> GGGFCTSAGALWIYPTNCPVRDYQLHISRAALFCNTLVCLPTGLGKTFIAAVVMYNFYRWFPSGKVVFMAPTKPLVTQQIEACYQVMGIPQSHMAEMTGSTQASTRKEIWCSKRVLFLTPQVMVNDLSRGACPAAEIKCLVIDEAHKALGNYAYCQVVRELVKYTNHFRILALSATPGSDIKAVQQVITNLLIGQIELRSEDSPDILTYSHERKVEKLIVPLGEELAAIQKTYIQILESFARSLIQRNVLMRRDIPNLTKYQIILARDQFRKNPSPNIVGIQQGIIEGEFAICISLYHGYELLQQMGMRSLYFFLCGIMDGTKGMTRSKNELGRNEDFMKLYNHLECMFARTRSTSANGISAIQQGDKNKKFVYSHPKLKKLEEVVIEHFKSWNAENTTEKKRDETRVMIFSSFRDSVQEIAEMLSQHQPIIRVMTFVGHASGKSTKGFTQKEQLEVVKQFRDGGYNTLVSTCVGEEGLDIGEVDLIICFDSQKSPIRLVQRMGRTGRKRQGRIVIILSEGREERIYNQSQSNKRSIYKAISSNRQVLHFYQRSPRMVPDGINPKLHK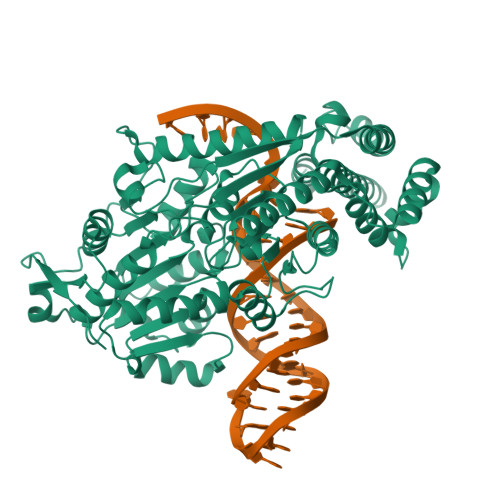MFITH>[2x]MGHHHHHHSGENLYFQGTIRSYKNLNLVRANIETESRQFIENKNYSIQSIGPMPGSRAGLRVVFTRPGVNLATVDIFYNGDGSTTIQYLTGANRSLGQELADHLFETINPAEFEQVNMVLQGFVETSVLPVLELSADESHIEFREHSRNAHTVVWKIISTSYQDELTVSL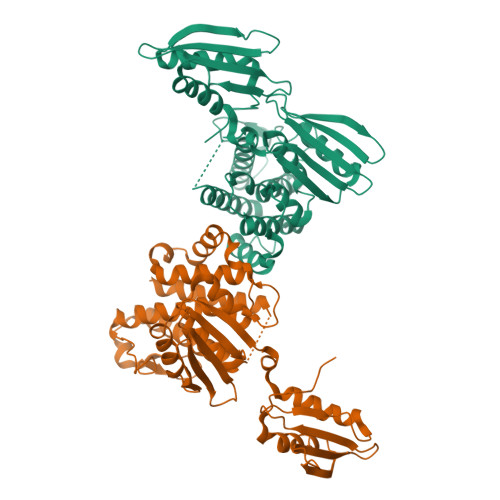HITTGKLQIQGRPLSCYRVFTFNLAALLDLQGLEKVLIRQEDGKANIVQQEVARTYLQTVMADAYPHLHVTAEKLLVSGLCVKLAAPDLPDYCMLLYPELATIEGVLKSKMSGLGMPVQQPAGFGTYFDKPAAHYILKPQFAATLRPEQINIISTAYTFFNVERHSLFHMETVVDASRMISDMARLMGKATRAWGIIKDLYIV The Vtc4p β-tunnel domain is not unique to eukaryotic polyP polymerases but is a structural hallmark of triphosphate tunnel metalloenzymes (TTMs), whose characteristic features are the presence of a topologically closed hydrophilic β-barrel, the preference for triphosphate-containing substrates, and for a divalent metal co-factor (PFAM families CYTH and VTC). Members of the ancient triphosphate tunnel metalloenzyme family can be found in all kingdoms of life. Our comparative analysis defines that most of these enzymes share a common catalytic mechanism in their tunnel centers, yet they have evolved different substrate recognition modes on their tunnel entries. The observed substrate plasticity apparently allows TTM proteins to act on a wide array of enzyme substrates and to perform very different reactions, many of which likely remain to be discovered.

We thus structurally characterized a mammalian TTM ThTPase, which was previously shown to specifically hydrolyze thiamine triphosphate (ThTP) into ThDP and Pi. We next solved a crystal structure of mouse ThTPase in the presence of ThTP and Mg2+ in a second crystal form grown at pH 9.0, where substrate hydrolysis can occur. Indeed, we found a product complex trapped in the active site of the enzyme, with a ThDP molecule and an orthophosphate located in the tunnel center. ThDP is coordinated by Arg-55 and Arg-57 in the substrate binding site but no longer allows for the coordination of a Mg2+/Mn2+ ion in metal binding site 1, possibly because the missing γ-phosphate would be required for Mg2+/Mn2+ coordination. The γ-phosphate in our structure apparently has been hydrolyzed, and the resulting Pi has slightly moved away from the tunnel center. It is now found coordinated by Arg-125 and in direct contact with a Mn2+ ion located in metal binding site 2, reinforcing the notion that this metal ion may play a crucial role in catalysis. The acidic patch in mouse ThTPase (corresponding to site 2 in AtTTM3 and ygiF) again allows for Mg2+ ion binding, as concluded from NMR titration experiments. The unique modes of substrate binding in ThTPases and adenylate cyclases allow these enzymes to carry out rather different reactions and to produce different leaving groups (ortho- and pyrophosphate, respectively) while maintaining a unified cleavage site in close proximity of metal binding site 2.

>GAMTQGLIEVERKFAPGPDTEERLQELGATLEHRVTFRDTYYDTSELSLMLSDHWLRQREGSGWELKCPGVTGVSGPHNEYVEVTSEAAIVAQLFELLGSGEQKPAGVAAVLGSLKLQEVASFITTRSSWKLALSGAHGQEPQLTIDLDSADFGYAVGEVEAMVHEKAEVPAALEKIITVSSMLGVPAQEEAPAKLMVYLQRFRPLDYQRLLEAASS[2x]>MALLPAVRRYGRLTRATGLVLEATGLQLPLGATCIIERQDGPETKEVESEVVGFNGQRLFLMPLEEVEGILPGARVYARNGHGDGLQSGKQLPLGPALLGRVLDGGGKPLDGLPAPDTLETGALITPPFNPLQRTPIEHVLDTGVRAINALLTVGRGQRMGLFAGSGVGKSVLLGMMARYTRADVIVVGLIGERGREVKDFIENILGPDGRARSVVIAAPADVSPLLRMQGAAYATRIAEDFRDRGQHVLLIMDSLTRYAMAQREIALAIGEPPATKGYPPSVFAKLPALVERAGNGIHGGGSITAFYTVLTEGDDQQDPIADSARAILDGHIVLSRRLAEAGHYPAIDIEASISRAMTALITEQHYARVRLFKQLLSSFQRNRDLVSVGAYAKGSDPMLDKAITLWPQLEAFLQQ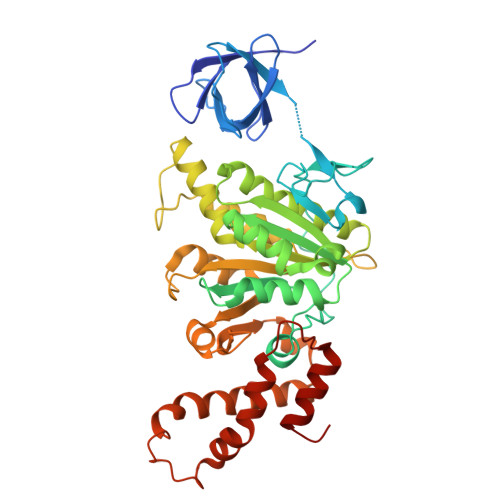GIFERADWEDSLQALDLIFPTV[2x]> XITID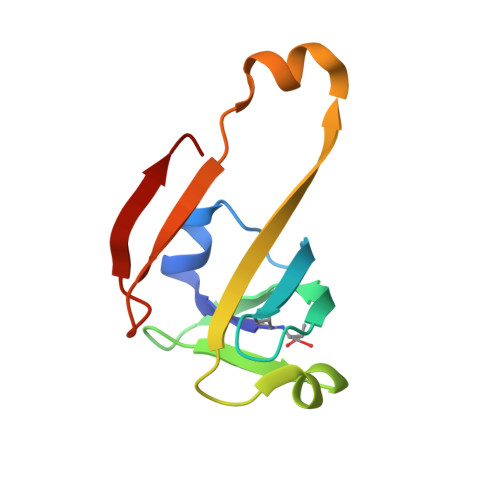EDLAKLAKLREGMKVEIVDVNNGERFSTYVILGKKRGEICVNGAAARKVAIGDVVIILAYASMNEDEINAHKPSIVLVDEKNEILEKGLEH>[26x]MFKALAGIVLALVATLAHAERIRDLTSVQGVRENSLIGYGLVVGLDGTGDQTTQTPFTTQTLNNMLSQLGITVPTGTNMQLKNVAAVMVTASYPPFARQGQTIDVVVSS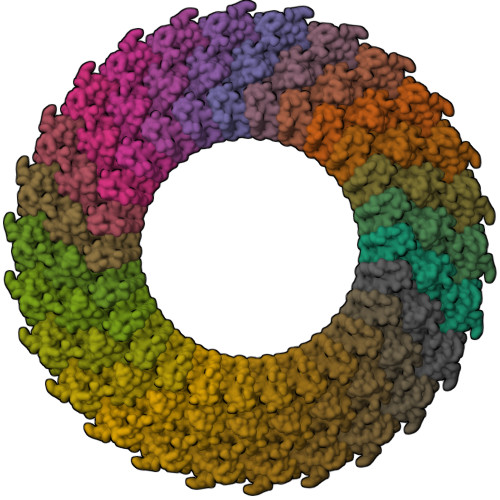MGNAKSLRGGTLLMTPLKGVDSQVYALAQGNILVGGAGASAGGSSVQVNQLNGGRITNGAIIERELPTQFGAGNTINLQLNDEDFTMAQQITDAINRARGYGSATALDARTVQVRVPSGNSSQVRFLADIQNMEVNVTPQDAKVVINSRTGSVVMNREVTLDSCAVAQGNLSVTVNRQLNVNQPNTPFGGGQTVVTPQTQIDLRQSGGSLQSVRSSANLNSVVRALNALGATPMDLMSILQSMQSAGCLRAKLEII> AQDDSTPDSLFAGLVGEYYGTNSQLNNISDFRALVDSKEADATFEAANISYGRGSSDVAKGTHLQEFLGSDASTLSTDPGDNTDGGIYLQGYVYLEAGTYNFKVTADDGYEITINGNPVATVDNNQSVYTVTHASFTISESGYQAIDMIWWDQGGDYVFQPTLSADGGS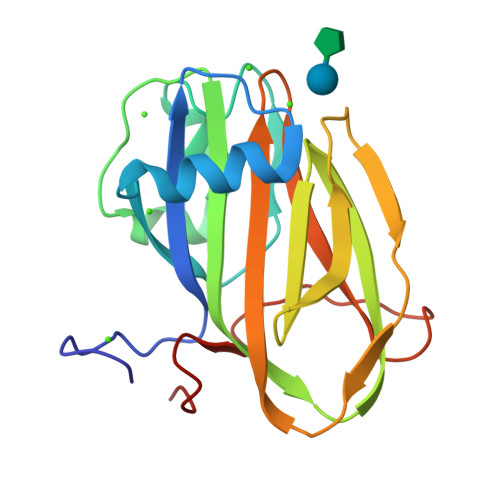TYFVLDSAILSSTGETPYTT> ANIVGGIEYSINNASLCSVGFSVTRGATKGFVTAGHCGTVNATARIGGAVVGTFAARVFPGNDRAWVSLTSAQTLLPRVANGSSFVTVRGSTEAAVGAAVCRSGRTTGYQCGTITAKNVTANYAEGAVRGLTQGNACMGRGDSGGSWITSAGQAQ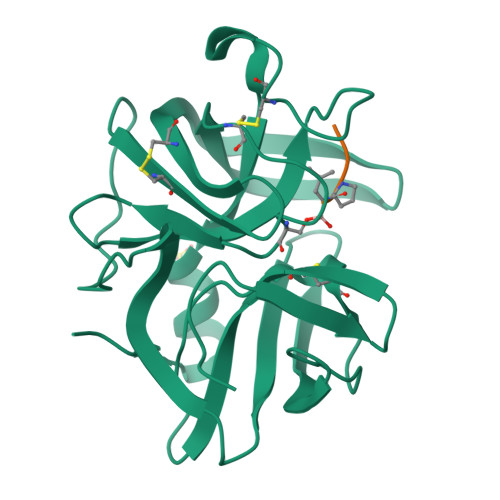GVMSGGNVQSNGNNCGIPASQRSSLFERLQPILSQYGLSLVTG;> XAAPL> PRGSHGKKRQRFVDKNGRCNVQHGNLGSEKRAETLMFSEHAVISMRDGKLTLMFRVGNLRNSHMVSAQIRCKLLKSRQTPEGEFLPLDQLELDVGFSTGADQLFLVSPLTICHVIDAKSPFYDLSQRSMQTEQFEVVVILEGIVETTGMTCQARTSYTEDEVLWGHRFFPVISLEEGFFKVDYSQFHATFEVP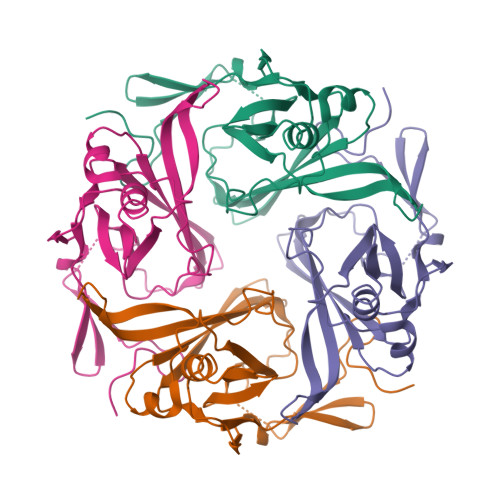TPPYSVKEQEEMLLMSSPL>GSHMLPSCKEDEYPVGSECCPKCSPGYRVKEACGELTGTVCEPCPPGTYIAHLNGLSKCLQCQMCDPAMGLRASRNCSRTENAVCGCSPGHF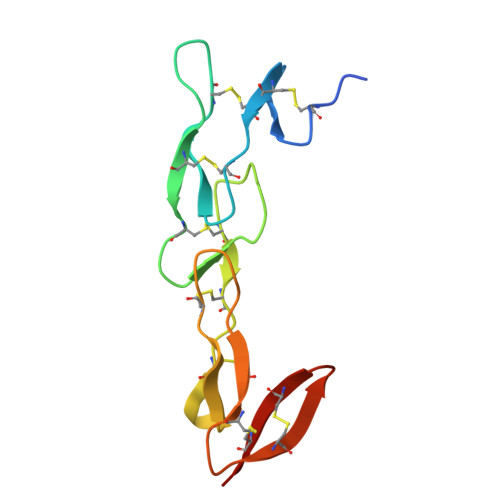CIVQDGDHCAACRAYA[2x]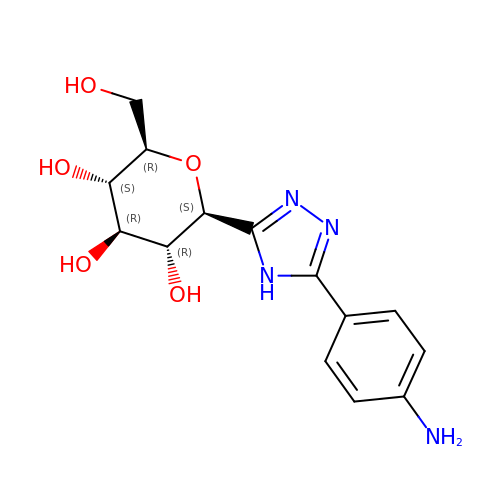(2~{S},3~{R},4~{R},5~{S},6~{R})-2-[5-(4-aminophenyl)-4~{H}-1,2,4-triazol-3-yl]-6-(hydroxymethyl)oxane-3,4,5-triol | C14 H18 N4 O5 | NDNZXPQRERAKKG-RMPHRYRLSA-N>GSTHWAFSPIQPGAARNMAAWQIAGKKDGPYQIDVSWPLTWSESGDASGKSANAVYLVDGNALFLTATETLRRRESHRPSETGTVVIAIGYPITDSVFSPRRSYDLTPPC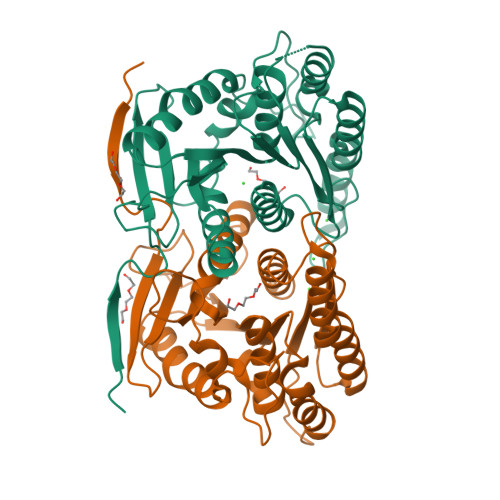DHYIPPEGPDGSPKPEAHGGADEFLTFIAEIVRPFVELKVFPRVSFGRTALFGHSYGGLFALHALFTKPSSFDVYLAASPSIWWNNRSILTEARRFISGAALFSSAHPVLRLSFGSREQYPVRQRVESDEMFKRRQRAAEQRRMNDNCEELYSELLASGRLCKLEVKEYLDEDHGSVIGPALSGGIMFLSNLSA[4x]Here we report the mechanism of three Fe(II)/α-ketoglutarate-dependent dioxygenases in bicyclomycin synthesis, which depicts the natural tactic to sequentially hydroxylate specific C−H bonds of similar substrates (cyclodipeptides). Three αKGDs (BcmE/BcmC/BcmG) catalyze site- and stereo-selective hydroxylation of inert C−H bonds in BCM’s (bicyclomycin) cyclic dipeptide scaffold (Fig. 1b3), one of the simplest peptide derivatives without additional functional groups. Our hypothesis posits distinct regulatory mechanisms: BcmE employs steric hindrance, BcmC relies on inherent reactivity, while BcmG utilizes a directing group to control C–H hydroxylation. Although these three enzymes share only 35–42% amino acid identities, the overall structures are similar, and r.m.s.d. values are 0.70 Å (SsBcmE vs SsBcmC), 1.07 Å (SsBcmE vs PaBcmG) and 0.87 Å (SsBcmC vs PaBcmG), respectively.

Except for solving the quaternary complex of PaBcmG•FeII•αKG•3, we did not get the other two complex structures using SsBcmE and SsBcmC. The DKP ring interacts with F248 via π-π stacking, while its two carbonyl groups form hydrogen bonds with T156 and S175, respectively. The 7-OH of 3 forms water-mediated hydrogen bonds with H154 and R81, whereas the 2’-OH group forms a hydrogen bond with the phenolic hydroxyl group of Y288 which couples with the amine group of Q94. Furthermore, the C-3’ is closer to the iron center, which is consistent with the result that BcmG catalyzed the C-3’ hydroxylation. Likewise, the comparison between PaBcmG•FeII•αKG and PaBcmG•FeII•αKG•3 structures revealed that the C-terminal helix may function as a gate or lid for the active pocket, and the binding of substrate triggers the closure of this gate. Our results suggest that the interactions between PaBcmG residues and substrate 3 control the substrate to be in a specific orientation for hydroxylation, which effectively reverses its inherent site selectivity. Combined with the crystal structure analyzes, we speculated that the hydrogen bonding interactions medicated by R281, Q94, H154, T156, S175 and Y288 and the hydrophobic interactions mediated by F96, F248, L280 and L284 stabilize and orient the substrate 3 in a suitable conformation to favor the C-3’ hydroxylation. Moreover, the hydrogen bonding interactions between Y288 (also interact with Q94) and 2’-OH drives C-3’ in substrate 3 to adopt a catalytically active conformation for hydroxylation. Collectively, we speculate that BcmG performs exquisite control over the site selectivity and stereoselectivity mainly through the directed guidance mediated by the hydrogen bond between Y288 and the 2’-OH of 3, similar to a directing group control strategy in chemical catalysis.

> MNPNATYALASAELIDGKLRFDSSDGFARAIADGFFFVKSPSLDLAAGDTFARNFYLPRQEGLGAPYQGFSQWTEDRLARREGYFSRDVDQVEQFFLESRFWQTVFPGPLLRQAERMRSFSLEVLRAVLAELDLPVELWDEATGRCLSMQGTYHLTFNHFRSHVRARGLNVHKDSGWVTILRSLEPGLEVLREGDWLPVSPRPGEFIVNFGCAMEILTRHSATPVAAVAHRVQEQLPGQADRFSYALFVDSSLDPRTCPGLFRYLPGHGLVLEADFEMFLNEILHNTYQENTQGLYLEHHHHHHHH6-{[(3R,4R)-4-(2-{[2-(2,3-difluorophenyl)-2,2-difluoroethyl]amino}ethoxy)pyrrolidin-3-yl]methyl}-4-methylpyridin-2-amine | C21 H26 F4 N4 O | 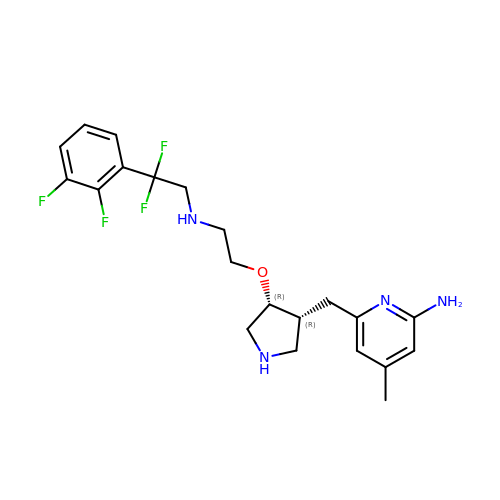SGDIVHJKRFAKAS-KDOFPFPSSA-N> GPGSIEVPSDDSVGLLAEPQVAMFCGKLNMHINVQSGKWEPDPTGTKSCISTKEGILKYCQEVYPDLQITNVVEANQPVSIQNWCKMGRRQCRSHTHIVVPYRCLVGEFVSDALLVPDKCKFLHQERMDMCESHLHWHTVAKESCGDRSMNLHDYGMLLPCGIDRFRGVEFVCCPMEEQK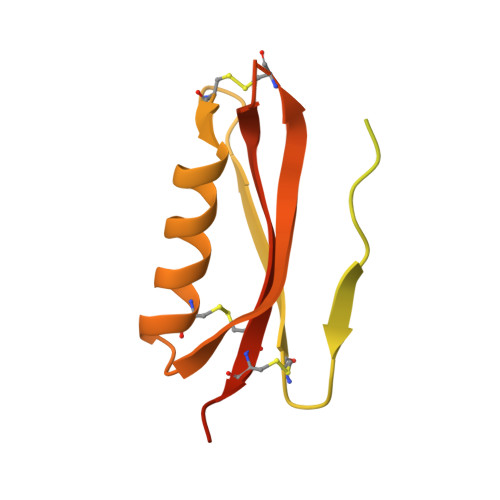DLDSEAAA>MSIVVKNNIHWVGQRDWEVRDFHGTEYKTLRGSSYNSYLIREEKNVLIDTVKHKFSREFVQNLRNEIDLADIDYIVINHAEEDHAGALTELMAQIPDTPIYCTANAIDSINGHHHHPEWNFNVVKTGDTLDIGNGKQLIFVETPMLHWPDSMMTYLTGDAVLFSNDAFGQHYCDEHLFNDEVDQTELFEQCQRYYANILTPFSRLVTPKITEILGFNLPVDMIATSHGVVWRDNPTQIVELYLKWAADYQEDRITIFYDTMYNNTRMMADAIAQGIAETD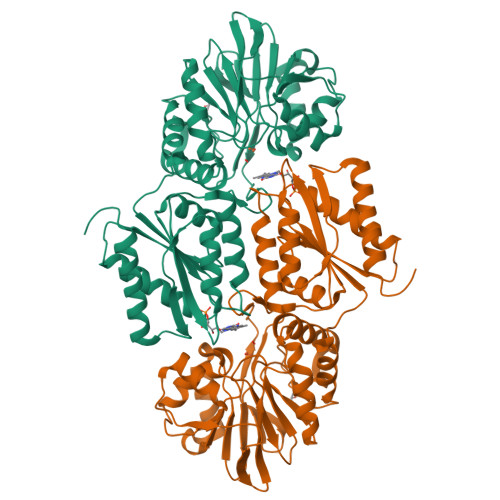PRVAVKIFNVARSDKNEILTNVFRSKGVLVGTSTMNNVMMPKIAGLVEEMTGLRFRNKRASAFGSHGWSGGAVDRLSTRLQDAGFEMSLSLKAKWRPDQDALKLCREHGREIARQWALAPLPQSTVNTVVKEETSATTTADLGPRMQCSVCQWIYDPAKGEPMQDVAPGTPWSEVPDNFLCPECSLGKDVFEELASEAK[2x]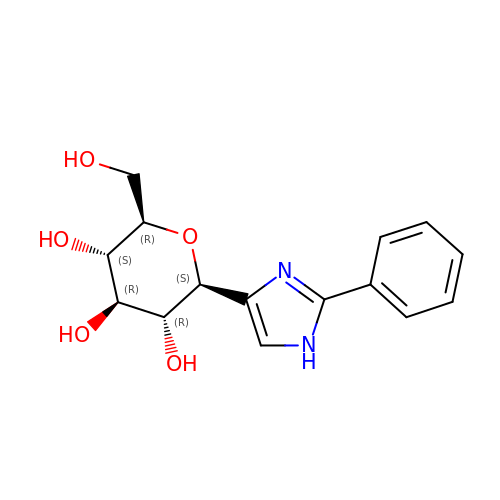(2~{R},3~{S},4~{R},5~{R},6~{S})-2-(hydroxymethyl)-6-(2-phenyl-1~{H}-imidazol-4-yl)oxane-3,4,5-triol | C15 H18 N2 O5 | HSTOUPNMEGVFOM-RGDJUOJXSA-N6-(4-methylsulfonylpiperazin-1-yl)-[1,2,4]triazolo[4,3-b]pyridazine | 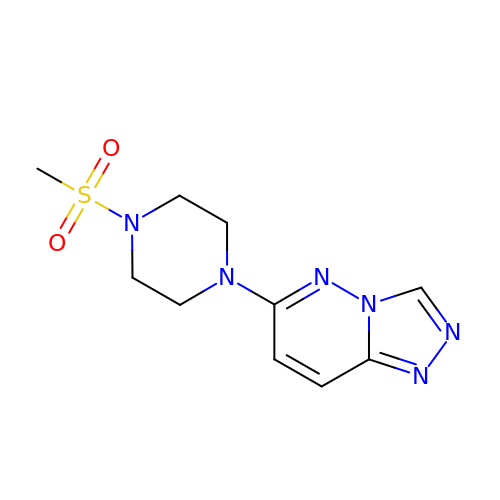C10 H14 N6 O2 S | UNYVOSROGSXTRY-UHFFFAOYSA-N>[4x]MKKTKIVCTIGPKTESEEMLAKMLDAGMNVMRLNFSHGDYAEHGQRIQNLRNVMSKTGKTAAILLDTKGPEIRTMKLEGGNDVSLKAGQTFTFTTDKSVIGNSEMVAVTYEGFTTDLSVGNTVLVDNGLIGMEVTAIEGNKVICKVLNNGDLGENKGVNLPGVSIALPALAEKDKQDLIFGCEQGVDFVAASFIRKRSDVIE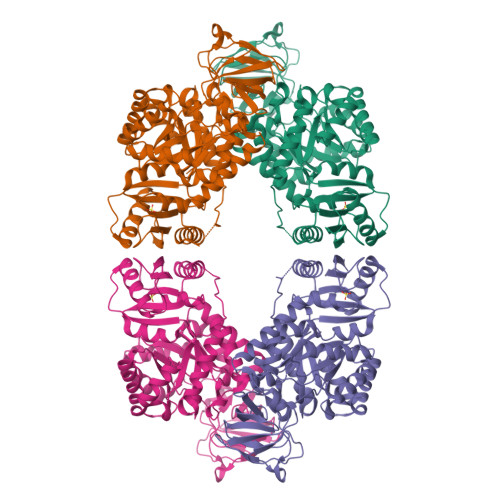IREHLKAHGGENIHIISKIENQEGLNNFDEILEASDGIMVARGDLGVEIPVEEVIFAQKMMIEKCIRARKVVITATQMLDSMIKNPRPTRAEAGDVANAILDGTDAVMLSGESAKGKYPLEAVSIMATICERTDRVMNSRLEFNNDNRKLRITEAVCRGAVETAEKLDAPLIVVATQGGKSARAVRKYFPDATILALTTNEKTAHQLVLSKGVVPQLVKEITSTDDFYRLGKELALQSGLAHKGDVVVMVSGALVPSGTTNTASVHVL> MAMSFEWPWQYRFPPFFTLQPNV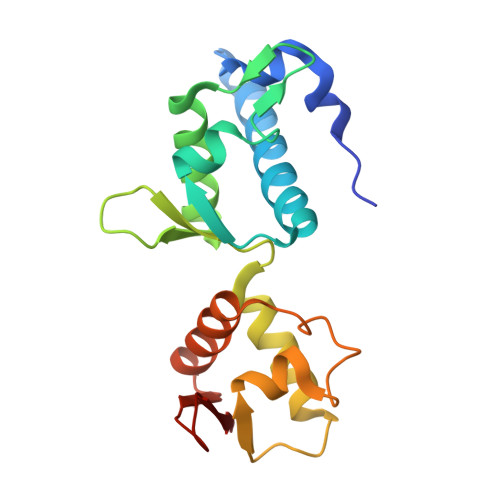DTRQKQLAAWCSLVLSFCRLHKQSSMTVMEAQESPLFNNVKLQRKLPVESIQIVLEELRKKGNLEWLDKSKSSFLIMWRRPEEWGKLIYQWVSRSGQNNSVFTLYELTNGEDTEDEEFHGLDEATLLRALQALQQEHKAEIITVSDGRGVKFF Adenoviruses are clinically important, both as human pathogens and as platforms for therapeutic applications. Species D adenovirus type 26 (HAdV-D26) is both a cause of EKC and other diseases and a promising vaccine vector. Here, we demonstrate that HAdV-D26 uses sialic acid–bearing glycans as a primary entry receptor and that this interaction can form a productive infection. We solve the structure of HAdV-D26K in complex with sialic acid [N-acetylneuraminic acid (Neu5Ac)], revealing a similar topology to the known sialic acid–interacting HAdV-D37 fiber knob in the sialic acid–binding pocket, but highlight crucial mechanistic differences likely to enhance HAdV-D26 affinity for sialic acid compared to other types.

We crystallized HAdV-D26K in complex with sialic acid to clarify the mechanism of interaction. Refinement of structures generated from HAdV-D26K crystals soaked in sialic acid shows electron density for a small-molecule ligand in the apical depression; this is best described by a racemic mixture of α and β anomers, in conjunction with double conformations of sialic acid. We observed three copies of sialic acid bound within the apex of the fiber knob trimer, as previously observed in HAdV-D37 and HAdV-D19p. The high resolution of the datasets generated to determine the sialic acid–bound HAdV-D26K structure enables visualization of multiple residue conformations with partial occupancy. We observe split density for Gln348 in both pH 8.0 and pH 4.0. While conformation A can form polar contacts with sialic acid, conformation B points into the solvent and cannot. We also observe greater occupancy of conformation A in the pH 8.0 structure (approximately 0.7), while at pH 4.0, the occupancy is evenly split. At pH 4.0, Gln348 has approximately half occupancy in each conformation. This implies the possibility of HAdV-D26K having lower sialic acid affinity under more acidic conditions, such as those encountered during endosomal trafficking down the lysosomal pathway.

> MRGSHHHHHHGSGDLVAWNKKDDRRTLWTTPDTSPNCKMSTEKDSKLTLTLTKCGSQVLGNVSLLAVTGEYHQMTATTKKDVKISLLFDENGILLPSSSLSKDYWNYRSDDSIVSQKYNNAVPFMPNLTAYPKPSAQNAKNYSRTKIISNVYLGALTYQPVIITIAFNQETENGCAYSITFTFTWQKDYSAQQFDVTSFTFSYLTQENKDKD>HHHHHIEGRHMAGPDRAELAELVRRLSVVHGRVTLSSGREADYYVDLRRATLHHRASALIGRLMRELTADWDYSVVGGLTLGADPVATAIMHAPGRPIDAFVVRKSAKAHGMQRLIEGSEVTGQRVLVVEDTSTTGNSALTAVHAVQDVGGEVVGVATVVDRATGAAEAIEAEGLRYRSVLGLADLGLD[2x]

The fifth step in the de novo biosynthetic pathway is catalyzed by the enzyme orotate phosphoribosyltransfrase that synthesises orotidine 5′-monophosphate (OMP) and pyrophosphate from α-D-5-phosphoribosyl-1-pyrophosphate (PRPP) and orotate (OA). Herein, we report the X-ray crystal structures of MtOPRT (coded by the rv0382c gene) in complex with PRPP, inorganic phosphate and an exogenous Fe(III) dicitrate molecule (ferric dicitrate, FDC) at 2.25 Å, 1.90 Å and 2.40 Å resolution, respectively. In all the structures herein described, both monomers composing the functional homodimeric unit are related by a 2-fold axis, with a solvent excluded surface between monomers of 1045 Å2 (13% of each subunit surface).

A PRPP molecule could be unambiguously identified in the active site in both monomers of the binary complex with the substrate crystallized in absence of Mg2+. Refinement statistics gave good correlation coefficient score (CC) for the PRPP molecule (CC = 0.89). 18, the three oxygens of the PRPP 5-phosphate group interact with the substrate pocket II (also defined as PRPP binding motif, residues 120–128) through a network of hydrogen bonds involving the amide group of the conserved residues Thr124 and Gly126 and the non-conserved residue Thr125. The ribose hydroxyl groups of the PRPP form hydrogen bonds interactions with Glu120 and Asp121. Glu120 contacts both the substrate O2′ and O3′, while Asp121 interacts only with the O2′. The PRPP pyrophosphate group occupies the substrate binding pocket I (residues 63–79) establishing a hydrogen bond between its O2β atom and the Nζ atom of Lys95, and a salt bridge between its O3β atom and the guanidino group of Arg38. The analysis of the enzyme structures in complex with PRPP and Pi lead to the identification of the molecular determinants responsible for ligand recognition and binding.> DPFTDDLEQYLDEKILRLKDEMNIAAQLDIDTLNKRIETGDTSLIAMQKVKLLPKVVSVLSKANLADTI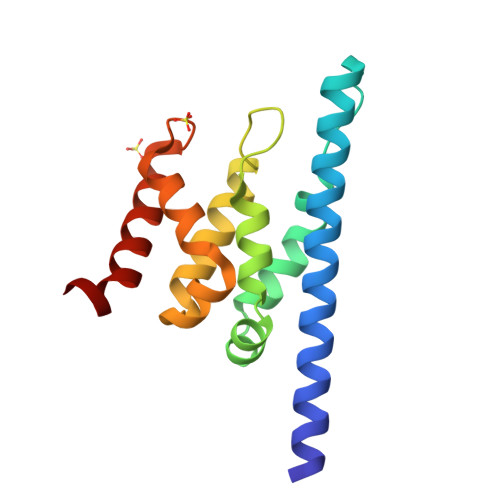LDNNLLQSVRIWLEPLPDGSLPSFEIQKSLFAALNDLPVKTEHLKESGLGRVVIFYTKSKRVEAQLARLAEKLIAEWTRPIIG> MGHHHHHHSHMRKIDLCLSSEGSEVILATSSDEKHPPENIIDGNPETFWTTTGMFPQEFIICFHKHVRIERLVIQSYFVQTLKIEKSTSKEPVDFEQWIEKDLVHTEGQLQNEEIVAH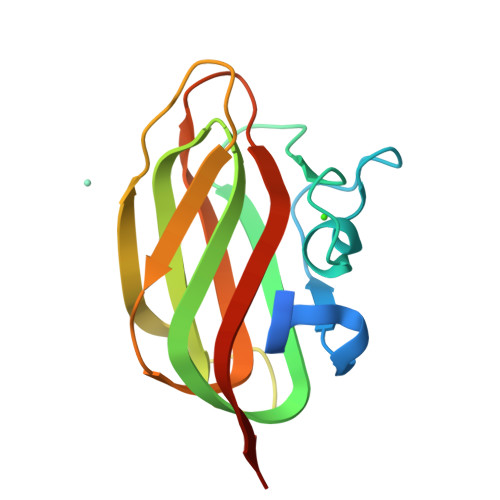GSATYLRFIIVSAFDHFASVHSVSAEGTVVSNLSS> MDSIQAEEWYFGKITRRESERLLLNAENPRGTFLVRESETTKGAYSLSVSDFDNAKGLNVKHYKIRKLDSGGFY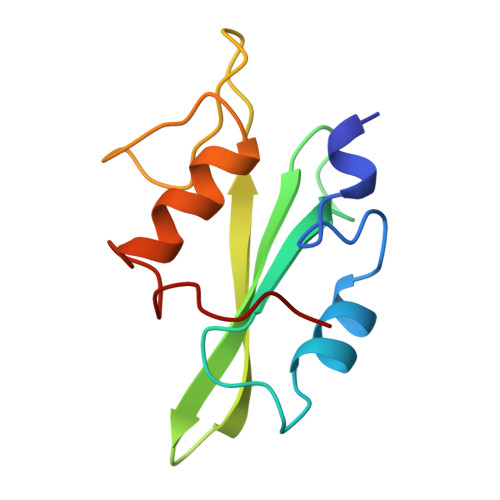ITSRTQFNSLQQLVAYYSKHADGLCHRLTTVCP> HHDITKVDTSGASEITARQDKLTLQGVDASHKLAEHDLVRMNKYKELITRVGQKHGLDPAIIAGIISRESRAGSALDHGWGDHGKGFGLMQVDKRYHKIVGAWDSEKHIS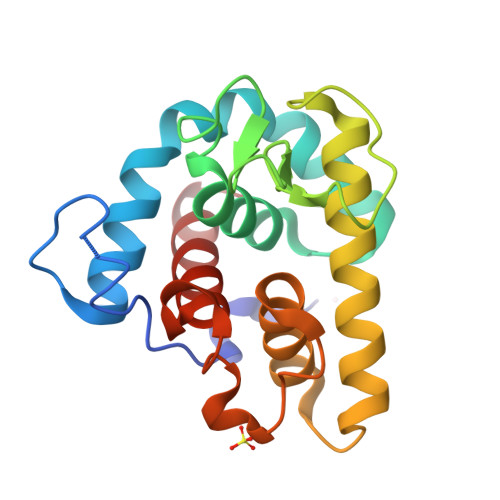QGTEILIEFIRRIQAKFPVWPKEHQLKGGISAYNAGDKNVRTYERMDVGTTGGDYSNDVVARSQWFKSQGY>[11x]MSLQGIHLSDLSYKHAILKESQYTIKRDVGTTTAVTPSSLQQEITLLCGEILYAKHADYKYAAEIGIQYISTALGSERVQQILRNSGSEVQVVLTRT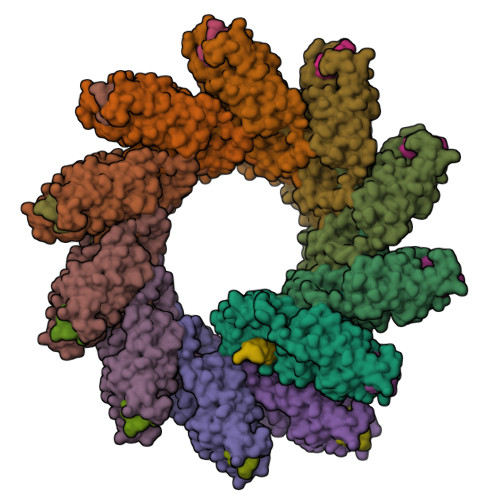YSLGKIKNNKGEDLQMLDIHGVEKSWVEEIDKEARKTMATLLKESSGNIPQNQRPSAPDTPIILLCVGALIFTKLASTIEVGLETTVRRANRVLSDALKRYPRMDIPKIARSFYDLFEQKVYHRSLFIEYGKALGSSSTGSKAESLFVNIFMQAYGAGQTMLRWGVIARSSNNIMLGHVSVQAELKQVTEVYDLVREMGPESGLLHLRQSPKAGLLSLANCPNFASVVLGNASGLGIIGMYRGRVPNTELFSAAESYAKSLKESNKINFSSLGLTDEEKEAAEHFLNVSDDSQNDYEKHHHHHH;>EDDIYQLIM[11x]>[2x]ITGYAACPRNWIGVGNKCFYFSEYASNWTFSQTFCKAQEAELARFDTEEELNFLSRYKGSFDYW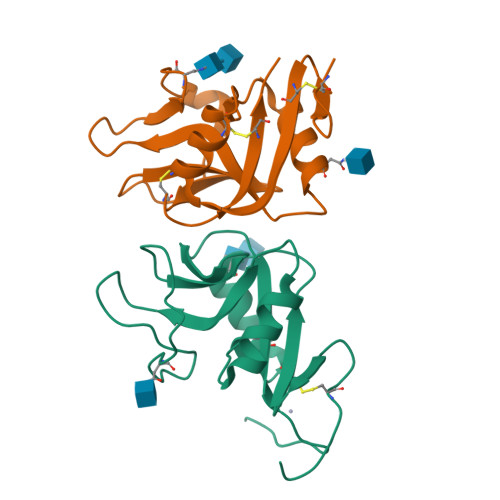IGLHRESSEHPWKWTDNTQYNYSLSIRGVERYAYLNDIGISSARVYADKRWSCSRLNSGTHHHHHHHHG;> GTGVQENRTKTTDSPAKLKCPKDWHSHQDKCFHVSQTSITWKGSLADCGGKGATLLLVQDQEELRFLRNLTKRISSSFWIGLSYTLSDEKWKWINGSTLNSDALNITGDTEKDSCASVSQDKVLSESCDSDNIWICQKELKRESTCNDSGT>[2x]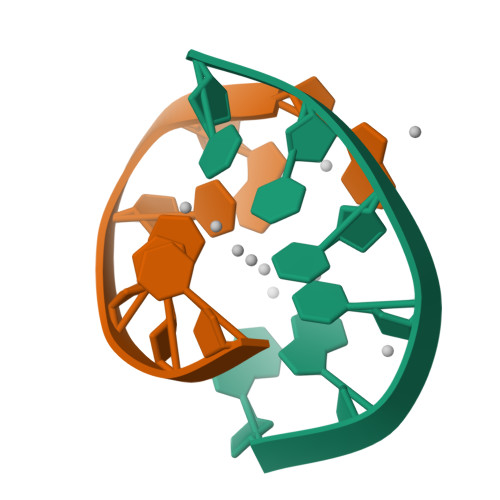AACCCC[AMINO (4-{(3AS,4R,8AS,8BR)-1,3-DIOXO-2- [3-(TRIMETHYLAMMONIO) 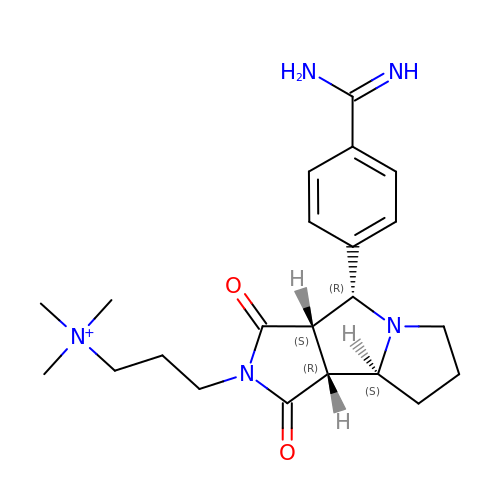PROPYL]DECAHYDROPYRROLO[3,4-A] PYRROLIZIN-4-YL}PHENYL) METHYLENE]AMMONIUM | C22 H32 N5 O2 | JCLUABDCGDTVPA-VJANTYMQSA-N>MSQEILNVEGM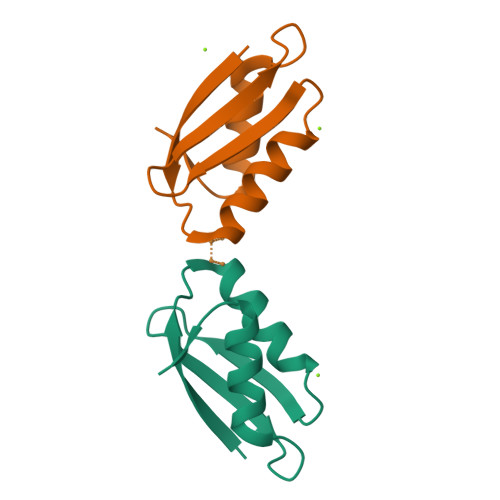SCGHCKSAVESALNNIDGVTSADVNLENGQVSVQYDDSKVAVSQMKDAIEDQGYDVV[2x]(E)-3,4-DIHYDROXY-N'-[(2-METHOXYNAPHTHALEN-1-YL)METHYLENE]BENZOHYDRAZIDE | C19 H16 N2 O4 | 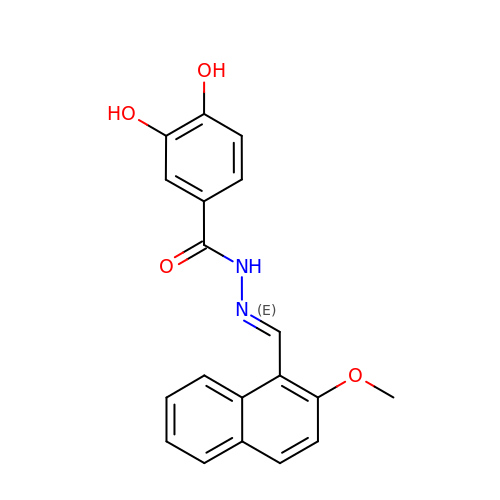TVOPERZEGKBKAY-RGVLZGJSSA-N>GLHCP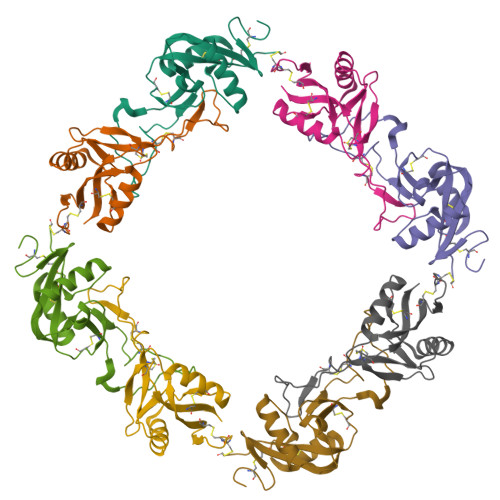SDWYYYDQHCYRIFNEEMNWEDAEWFCTKQAKGAHLVSIKSAKEADFVAWMVTQNIEESFSHVSIGLRVQNKEKQCSTKWSDGSSVSYDNLLDLYITKCSLLKKETGFRKWFVASCIGKIPFVCKFPPQC[2x];>[2x]GFCCPSHWSSYDRYCYKVFKQEMTWADAEKFCTQQHTGSHLVSFHSTEEVDFVVKMTHQSLKSTFFWIGANNIWNKCNWQWSDGTKPEYKEWHEEFECLISRTFDNQWLSAPCSDTYSFVCKFEA>[2x]MTIRNQRFSLLKQPISSTLNQHLVDYPTPSNLSYWWGFGSLAGICLVIQIVTGVFLAMHYTPHVDLAFNSVEHIMRDVEGGWLLRYMHANGASMFFIVVYLHIFRGLYYASYSSPREFVWCLGVVIFLLMIVTAFIGYVLPWGQMSFWGATVITSLASAIPVVGDTIVTWLWGGFSVDNATLNRFFSLHYLLPFILVGASLLHLAALHQYGSNNPLGVHSEMDKIAFYPYFYVKDLVGWVAFAIFFSIWIFYAPNVLGHPDNYIPANPMSTPPHIVPEWYFLPIYAILRSIPDKAGGVAAIALVFICLLALPFFKSMYVRSSSFRPIYQGMFWLLLADCLLLGWIGCQPVEAPFVTIGQISSLVFFLFFAITPILGRVGRGIPNSYTDETDHT;>MLRVAGRRLFSVSQRSSTATSFVVSRDHTLSDGGGDSSSAPRSLPSADLSSYHRSLIRGFSSQVLAQGNEIGFGSEVPATVEAVKTPNSKIVYDDHNHERYPPGDPSKRAFAYFVLSGGRFVYASVLRLLVLKLIVSMSASKDVLALASLEVDLGSIEPGTTVTVKWRGKPVFIRRRTEDDIKLANSVDVGSLRDPQEDSVRVKNPEWLVVVGVCTHLGCIPLPNAGDYGGWFCPCHGSHYDISGRIRKGPAPYNLEVPTYSFLEENKLLIG[2x];>MVGGGVIRQLLRRKLHSQSVATPVLSWLSSKKANEDAGSAGLRAFALMGAGITGLLSFSTVASADEAEHGLECPNYPWPHEGILSSYDHASIRRGHQVYQQVCASCHSMSLISYRDLVGVAYTEEEAKAMAAEIEVVDGPNDEGEMFTRPGKLSDRLPEPYSNESAARFANGGAYPPDLSLVTKARHNGQNYVFALLTGYRDPPAGISIREGLHYNPYFPGGAIAMPKMLNDEAVEYEDGTPATEAQMGKDVVSFLSWAAEPEMEERKLMGFKWIFLLSLALLQAAYYRRLKWSVLKSRKLVLDVVN[2x];>MGKQPVKLKAVVYALSPFQQKIMTGLWKDLPEKIHHKVSENWISATLLVTPVVGTYWYAQYFKEQEKLEHRF[2x];>[2x]MADDEVVDPKKYLEESCKPKCVKPLLEYQACVKRIQGDDSGHKHCTGQYFDYWQCIDKCVAPKLFAKLK;>MEYAARRNQKGAFEGFYKLIMRRNSVYVTFIIAGAFFGERAVDYGVHKLWERNNVGKRYEDISVLGQRPVEE[2x];>[2x]MAGTSGLLNAVKPKIQTIDIQAAAGWGIAAAAGAIWVVQPFGWIKKTFIDPPPTEEK

Protein complexes of the mitochondrial respiratory chain assemble into respiratory supercomplexes. Here we present the high-resolution electron cryo-microscopy structure of the Arabidopsis respiratory supercomplex consisting of complex I and a complex III dimer, with a total of 68 protein subunits and numerous bound cofactors. A complex I-ferredoxin, subunit B14.7 and P9, a newly defined subunit of plant complex I, mediate supercomplex formation. We propose that the main role of the plant supercomplex is to stabilize its components in the membrane.

Our 2 Å structure now shows the bound, co-purified Q substrate in each of the two Qo sites of the complex III dimer and surrounding water molecules in close-to-atomic detail. Both Rieske head domains assume the b-state, with the Rieske FeS cluster positioned 6.8 Å away from the bound Qo, and the FeS-coordinating H237 of the Rieske domain interacting with the Qo head group via a 2.9 Å hydrogen bond. In this distal binding position relative to haem bL, electrons can easily pass from Qo to the Rieske iron–sulphur cluster in the course of the Q cycle. During the cycle, protons from the quinol are released to the cristae lumen. In our structure, as in the stigmatellin- and HHDBT-bound yeast complex, one proton can be directly transferred to H237 of the Rieske head domain. The second proton can escape via a short chain of water molecules to Cyt b H259 and then to the cristae lumen. An alternative, longer path would lead via Cyt b Y280 and the bL propionate group to a water cluster surrounded by conserved polar residues of Cyt b (R85, Y86, N90, N255, Y263 and N262). Either pathway would enable proton release to the bulk solvent without involving Cyt b E278 in the Qo motif. However, in the Arabidopsis supercomplex, E278 does not interact with Qo and only contributes to a water chain via its backbone nitrogen atom.[METHYLTHIO]ACETATE | C3 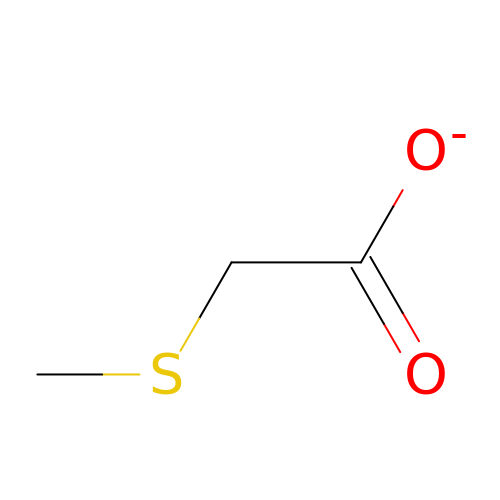H5 O2 S | HGTBAIVLETUVCG-UHFFFAOYSA-M>AAASMDAVTAEKFSPASFLDKKETGVL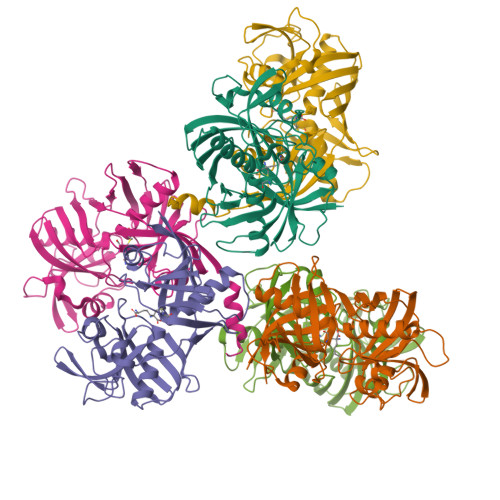HFVKYHGLGNDFILVDNRDSSEPKITQEQAAKLCDRNFGVGADGVIFAMPGVNGTDYAMRIFNSDGSEPEMCGNGVRCFARFIAELENLQGKHSFTIHTGAGLIVPEIQDDGQVKVDMGTPILKAQDVPTKLSGNKGEAVVEAELVVDGVSWNVTCVSMGNPHCITFGKKGGPNLKVDDLNLPEIGPKFEHHEMFPARTNTEFVEVLSRSHLKMRVWERGAGATLACGTGACALVVAAVLEGRADRKCTVDLPGGPLEIEWKQEDNHIYMTGPAEAVFYGSALLHHHHHH[6x]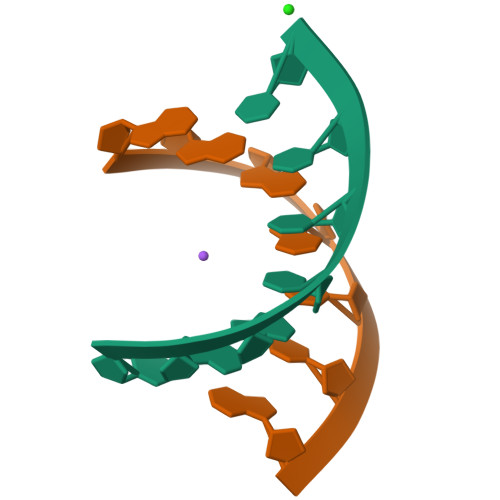>[2x]UAGCUCC;>GGGGCUA[2x]> 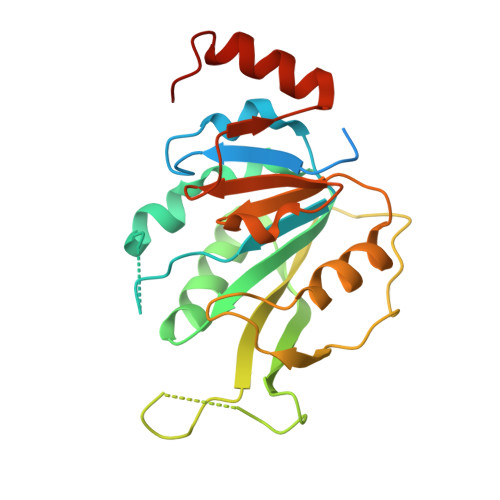MGHHHHHHSSGRENLYFQGALTQSVGGDSSADRLFPPQWICCDIRYLDVSILGKFAVVMADPPWDIHMELPYGTLTDDEMRRLNIPVLQDDGFLFLWVTGRAMELGRECLNLWGYERVDEIIWVKTNQLQRIIRTGRTGHWLNHGKEHCLVGVKGNPQGFNQGLDCDVIVAEVRSTSHKPDEIYGMIERLSPGTRKIELFGRPHNVQPNWITLGNQLDGIHLLDPDVVARFKQRYPDGIISKPKNL N-[1-[(2R,3S,4R,5R)-5-(6-aminopurin-9-yl)-3,4-dihydroxyoxolan-2-yl]propan-2-yl]-5-(4-fluorophenyl)-2,3-dihydroxybenzamide 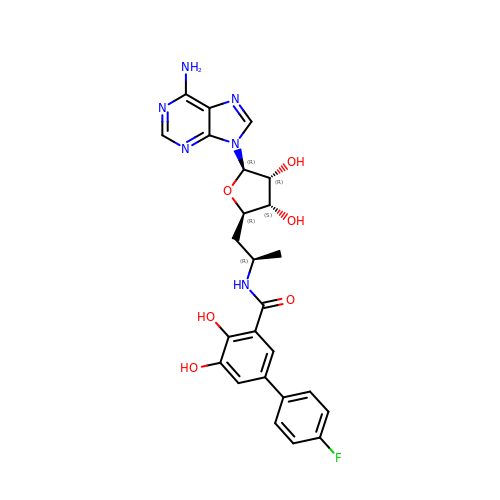| C25 H25 F N6 O6 | PQAIDYIFCYLFAS-RGJCZRFTSA-N>[2x]MVLYFIG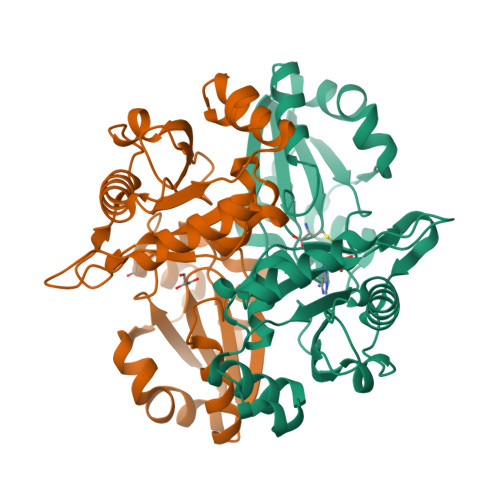LGLYDERDITVKGLEIAKKCDYVFAEFYTSLMAGTTLGRIQKLIGKEIRVLSREDVELNFENIVLPLAKENDVAFLTPGDPLVATTHAELRIRAKRAGVESYVIHAPSIYSAVGITGLHIYKFGKSATVAYPEGNWFPTSYYDVIKENAERGLHTLLFLDIKAEKRMYMTANEAMELLLKVEDMKKGGVFTDDTLVVVLARAGSLNPTIRAGCVKDLIREDFGDPPHILIVPGKLHIVEAEYLVEIAGAPREILRVNV>GSSGDKITVHFINRDGETLTTKGKIGDSLLDVVVQNNLDIDGFGACEGTLACSTCHLIFEQHIFEKLEAITDEENDMLDLAYGLTDRSRLGCQICLTKAMDNM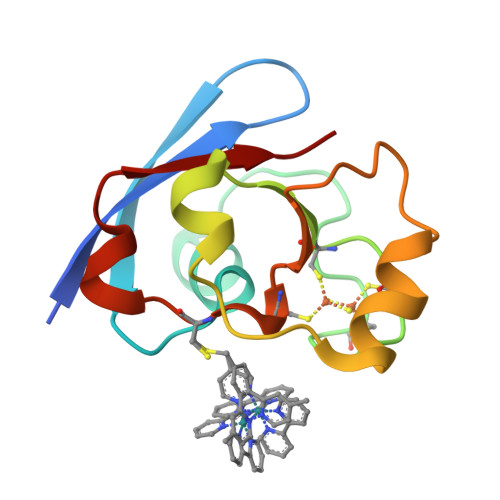TVRVP[2x]1-phenyl-5-propan-2-ylsulfanyl-1,2,3,4-tetrazole 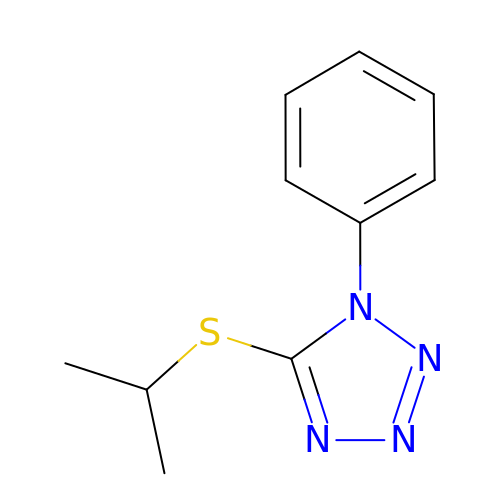| C10 H12 N4 S | SRXNAOIEUJQDHS-UHFFFAOYSA-N> VIASVEDGGDGDTSKDDWLWYKQPASQTDATATAGGNYGNPDNNRWQQTTLPFGNGKIGGTVWGEVSRERVTFNEETLWTGGPGSSTSYNGGNNETKGQNGATLRALNKQLANGAETVNPGNLTGGENAAEQGNYLNWGDIYLDYGFNDTTVTEYRRDLNLSKGK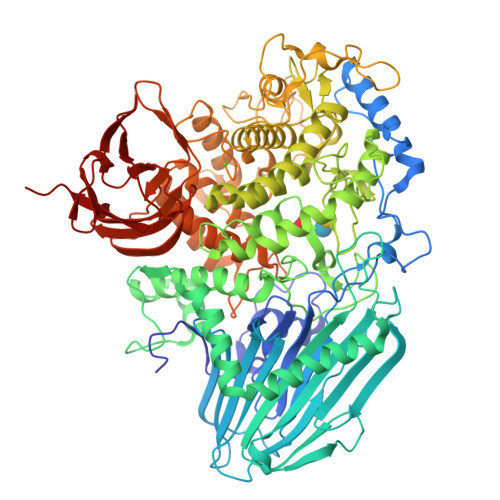ADVTFKHDGVTYTREYFASNPDNVMVARLTASKAGKLNFNVSMPTNTNYSKTGETTTVKGDTLTVKGALGNNGLLYNSQIKVVLDNGEGTLSEGSDGASLKVSDAKAVTLYIAAATDYKQKYPSYRTGETAAEVNTRVAKVVQDAANKGYTAVKKAHIDDHSAIYDRVKIDLGQSGHSSDGAVATDALLKAYQRGSATTAQKRELETLVYKYGRYLTIGSSRENSQLPSNLQGIWSVTAGDNAHGNTPWGSDFHMNVNLQMNYWPTYSANMGELAEPLIEYVEGLVKPGRVTAKVYAGAETTNPETTPIGEGEGYMAHTENTAYGWTAPGQSFSWGWSPAAVPWILQNVYEAYEYSGDPALLDRVYALLKEESHFYVNYMLHKAGSSSGDRLTTGVAYSPEQGPLGTDGNTYESSLVWQMLNDAIEAAKAKGDPDGLVGNTTDCSADNWAKNDSGNFTDANANRSWSCAKSLLKPIEVGDSGQIKEWYFEGALGKKKDGSTISGYQADNQHRHMSHLLGLFPGDLITIDNSEYMDAAKTSLRYRCFKGNVLQSNTGWAIGQRINSWARTGDGNTTYQLVELQLKNAMYANLFDYHAPFQIAGNFGNTSGVDEMLLQSNSTFTDTAGKKYVNYTNILPALPDAWAGGSVSGLVARGNFTVGTTWKNGKATEVRLTSNKGKQAAVKITAGGAQNYEVKNGDTAVNAKVVTNADGASLLVFDTTAGTTYTITKKAS>[2x]MPVPNP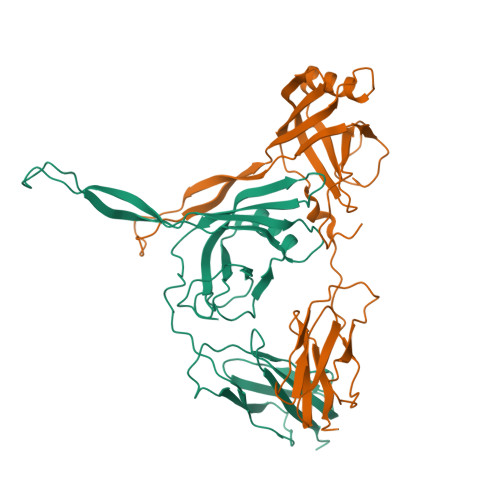TMPVKGAGTTLWVYKGSGDPYANPLSDVDWSRLAKVKDLTPGELTAESYDDSYLDDEDADWTATGQGQKSAGDTSFTLAWMPGEQGQQALLAWFNEGDTRAYKIRFPNGTVDVFRGWVSSIGKAVTAKEVITRTVKVTNVGRPSMAEDRSTVTAATGMTVTPASTSVVKGQSTTLTVAFQPEGVTDKSFRAVSADKTKATVSVSGMTITVNGVAAGKVNIPVVSGNGEFAAVAEITVTAS> MAPSADITSSGPSDASKPLAGKVALTTGAGRGIGRGIAIELGRRGASVVVNYGSSSKAAEEVVAELKKLGAQGVAIQADISKPSEVVALFDKAVSHFGGLDFVMS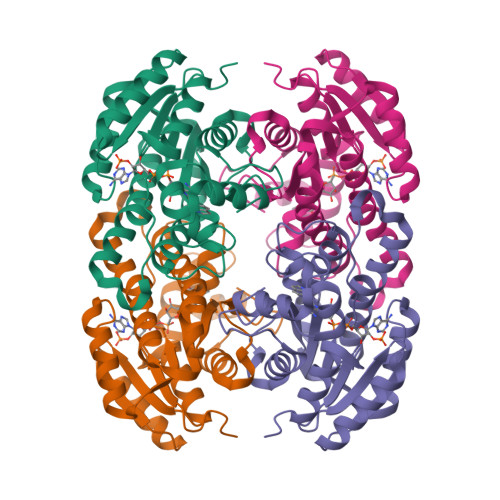NSGMEVWCDELEVTQELFDKVFNLNTRGQFFVAQQGLKHCRRGGRIILTSSIAAVMTGIPNHALYAGSKAAVEGFCRAFAVDCGAKGVTVNCIAPGGVKTDMFDENSWHYAPGGYKGMPQEKIDEGLANMNPLKRIGYPADIGRAVSALCQEESEWINGQVIKLTGGGI>[3x]ELDYEPAHISLDPQTSHPKLLLSEDHQRAQFSYK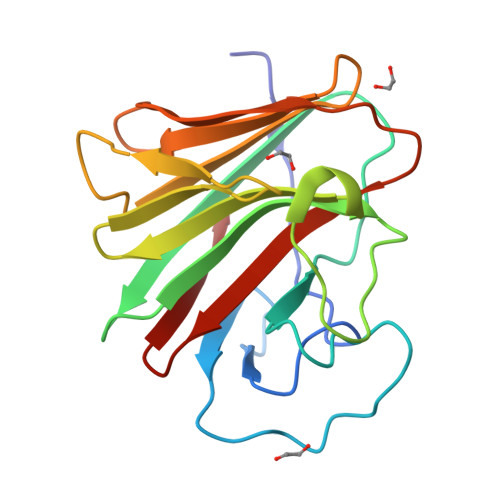WQNSPDNPQRFDRATCVLAHTGITGGRHTWVVSIDLAHGGSCTVGVVSEDVQRKGELRLRPEEGVWAVRLAWGFVSALGSFPTRLTLKEQPRQVRVSLDYEVGWVTFTNAVTREPIYTFTASFTRKVIPFFGLWGRGSSFSLSS(1~{R},2~{R},3~{R},4~{S},6~{S})-6-azanyl-2,3,4-tris(oxidanyl)cyclohexane-1-carboxylic 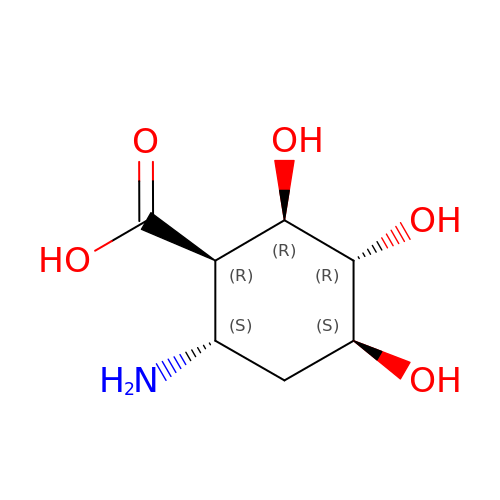acid | C7 H13 N O5 | DNFVBIRHFDBCAW-HGVZOGFYSA-N>[5x]PPPIADEPLTVNTGIYLIESYSLDDCAETFKVNAFLSLSWKDRRLAFDPVRSGVRVKTYEPE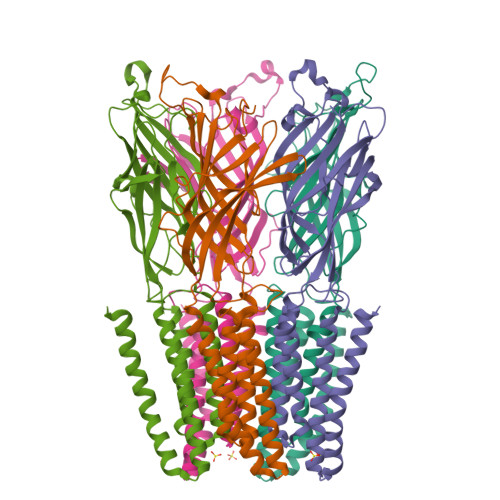AIWIPEIRFVNVENARDADVVDISVSPDGTVQYLERFSARVLSPLDFRRYPFDSQTLHIYLIVRSVDTRNIVLAVDLEKVGKNDDVFLTGWDIESFTAVVKPANFALEDRLESKLDYQLRISRQYFSYIPNIILPMLFILFISWTAFWSTSYEANVTLVVSTLAAHIAFNILVETCLPKTPYMTYTGAIIFMIYLFYFVAVIEVTVQHYLKVESQPARAASITRASRIAFPVVFLLANIILAFLFFGF>[35x]FTLIELMIVIAIVGILAAVALPAYQDYTARAQVSEAILLAEGQKSAVTEYYLNHGKWPENNTSAGVASSPTDIKGKYVKEVEVKNGVVTATMLSSGVNNEIKGKKLSLWARRENGSVKWFCGQPVTRTDDDTVADAKDGKEIDTKHLPSTCRDNFDAK;>[6x]MSGRLGELLVRENLISVQQLRKAQEEQQKNGTRIGTALVKTGAIEESKLTDFLSKQYGVPAINLKDFDVEPDIIKLVPKEVAEKHLVVPVNRAGPSLIVAMCDPSNIFAVDDLKFLTGYNIETVVASEVSIREAIERYYAEKGPSLEDIVGDVGDDIEVTKEETENIDEMAKAADDAPVVKLVNLILMDAIKKRASDIHVEPYEKDFRVRFRIDGVMYEVMRPPMKLRNAITSRLKIMASLDISERRLPQDGRIKIKMGGGKEMDFRVSVCPTLFGEKVVMRLLDKSNLQLDMTKLGFDAQPLAWFKEAIDRPYGMVLVTGPTGSGKTTTLYSALSSLNGLDTNICTAEDPVEFNFAGINQVQMHDDIGLNFAAALRSFLRQDPDIIMIGEIRDFETAEIGVKAALTGHLVLSTLHTNDAPGTVSRLLNMGIEPFLVTASLNLILAQRLARRLCPACKKPAENVDEQALIDAGVPPDKIGTFTMYEKVGCRDCNDRGYRGRVAIYEVMPFWDGLKELVINGASAAELKQEAIRLGMSSLRMSGLRKMMDGATTLEEVVGNTAPDRF;>[2x]MAAPAVKSASTPKKATAQFLWEAKTKSGESKKGEMEAMDVEAVNARLKSLGLNPVKVRKKSMLDGDITIPGFGGVEGKDILVFTRQFATMIDAGLPLVQCLDILASQMDNPSFKKVLFAIKSKVEQGSTFADALKEHPKVFDELYVQLCAAGEVGGILDAILNRLAAYREKNEKLKSKVKSAMTYPIIVILVAIGVTAVLLLKVTPVFEKMFADFGSELPGPTQMIVNFSHMAQEYFFHVAGSIVAVVMSFTWSYRQPRGRKFWDKVFLFMPVFGPVLRKVAVARFTRTLGTMISSGVPILDALDVTAKTAGNRTVEDAIIYVRGKIAEGKNIAGPLAETKVFPSMVVQMIGVGEATGAMDTMLNKIADFYDDEVDAAINSLTAMIEPVLMVFLGGVVGGFLIGMYLPIFSLAGAIQ;>[12x]MVRGSRPSGGQAGSRHFLGGVDGQCYAGCLSTESRMAKGKLVLGLDIGSTSIKMILLKEQRKRGEVIYALQSFGMKPLPPEAIVDGALMNSTAIVQAVQDLMSELKVKGKDVAIGVSGHSVIIKKIQMPRMSQDELEESIQWEAEQYIPFDVKDVNIDTQILDGGGNDATGQMDVLLVAAKKDMINDYTTVVSEAGLAPVVVDVDAFAVQNMFSVNYDVPERETVVLINAGASVVNINIISNGATVFTRDVTIGGNQFTEEIQKQLNVSYEEAEALKIGGNGAD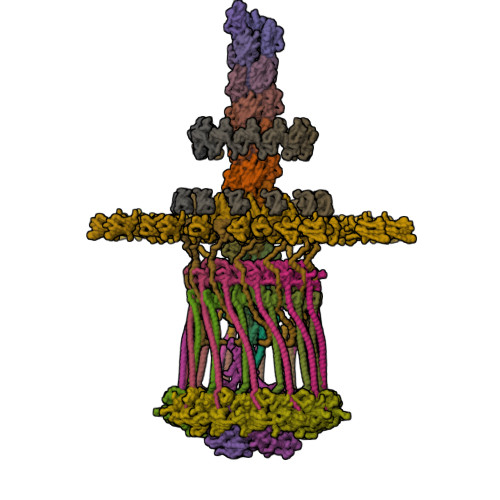ADAVVPQDVERVLSSVAEQVAGEIQRSLDFYAGTAADSNFSKVYLSGGTAKIPALFKTIEARTGVPVEILNPFRKIEVDNRKFDPAFVMDVAPMAAVAVGLALRRPGDKLA;>[12x]MMIRINLLPVRAVKKREMGRQVLVLFAVVLIGAGVANYLWYDDRQSELEAHQAGVASTKARIAELEKIIGEVKNINTRKAEVEKKLAVLDALRKGRSGPVRMMDALASATPKKVWVKTFSENNNAVSIDGSAVSHDEVAEFMRGLNGVVWTPKGMGRLVDRRRDSKTARVEMLTSDATIEEFPEAQVSPFFKNIDLQTAKQVGGAQVGVPILVEFKITMTSNYAI;>MDKYLDQFVKAPPAIKFGGLAFVVGALTAANFFMVIQPTEEEIGWAVAERRKLDLELADKSEIAQNLNERRREMDVLEQKLSEALTELPEQRDIEELLAQINDIGKKSGLELSSVTPGKESVGGGEFFARIPIKMTVSGNYHEIALFLQEMANMRRIVNVNNIKFDSAKLKNEKVVLQSEFQATTFRFVEQKAAASTAGNSNSKK[12x];>MLAACEEPPAPAPPPAKPKAAAAVPVKAAPTETGAQAAPSYSYVYNPVGKRDPFRSPIDELGPVNANPVAACNEPLCSFDLDQLKLVAVVTGDASPVAMVEDPAGRGHIVRRNTRMGRQGGKVTQILRDSVTVTEVFSGNGEIIKNPVTLQLKPDAKQDPAYNMMTGRNYGE[12x];>MLEESAVTRGKWMLAAAWAVVLVGARVHGAELNTLRGLDVSRTGSGAQVVVTGTRPPTFTVFRLSGPERLVVDLSSADATGIKGHHEGSGPVSGVVASQFSDQRASVGRVLLALDKASQYDVRADGNRVVISVDGTSQSVDAKRAETPARTERMTASVEAKPHPVAAQAPAKVVKAESAAVPKAALPENVVAAEADEREVSNPAQHITAMSFADDTLSIRADGDIARYEVLELADPPRLAVDLFGVGLATRAPRVKSGALRDVRVGAHADKVRLVLDVRGTMPAYRVDRANRGLEVVLGRAVARTWRRPLRPRAVVASVAEVEPLRQTPVKSDASPVVEVKDVRFEESSSGGRIVMKLSGTSGWKVDRPDPRSAVLTLDNARLPKKFERSLDTSALDTPVKMISAFSVPGAGGKVRLVVAADGAIEEKVSQSAGTLSWRLDVKGVKTEEVAVAQRTAGFTTEAPAYAAEGAPQQARYRGKRVSFEFKDIDIQNLLRVIAEISKKNIVVADDVSGKVTIRLRNVPWDQALDLVLRTKALGKEEFGNIIRIAPLKTLEEEARLRQERKKSLQQQEDLMVNLLPVNYAVAADMAARVKDVLSERGSVTVDQRTNVLIVKDVRSNTERARSLVRSLDTQTPQVLIESRIVEANTSFSRSLGVQWGGQARAGQATGNSTGLIFPNNLAVTGGVTGTGAGLPDNPNFAVNLPTGTGQGVGGAMGFTFGSAGGALQLNLRLSAAENEGSVKTISAPKVTTLDNNTARINQGVSIPFSQTSAQGVNTTFVEARLSLEVTPHITQDGSVLMSINASNNQPDPSSTGANGQPSIQRKEANTQVLVKDGDTTVIGGIYVRRGATQVNSVPFLSRIPVLGLLFKNNSETDTRQELLIFITPRILNRQTIAQTL[12x];>[12x]MMLLSKGRPAMRSRILTSLMLSLAVAPTAYAQQENEEEQDTGGEMGGAEVMDEAPDSAPPTSVAMPPGAPRGRESAPGEVHSVESGDTLWDLSQRYLGSPWYWPKVWSYNPEIANPHWIYPGNQVRFFAAGEEVPTQVTEMVVDEGDVTAPMEMTSNDQVIVTGKIGVDLANSVPVTTQGFVTQRELDEAGRIEGSPSNAVMLSFPDSVYVRFKRKGDVKVGDRYVVYHTTQAVKHPVTGRPLGFLTDFVGTLRVQRVGDGIVTAQIMDTWDGIERGDLVGPVGERLTERVAPKPNAKQVDGTVITALVPYLTVLGENHSIVVDKGSADGVELGNTFNILRKGDPSRHVLGHDVRKPSKEEQSFPWRSIGACMVTEVKERTSNCLMTRSLEELVPGDRAHMSAGASPSASR>[2x]MGSSHHHHHHSSG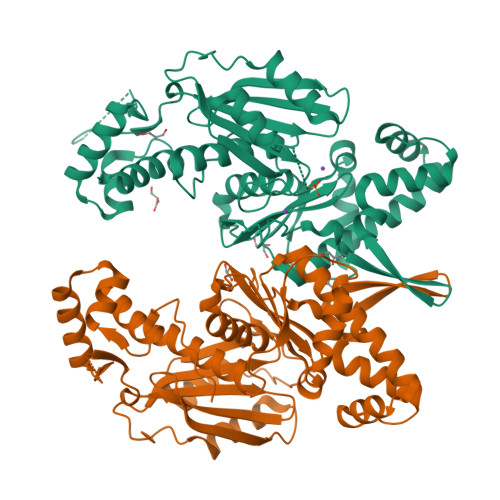ENLYFQGPMNDNEKRVLREIYNHHNISRTQISKNLEINKATISSILNKLKYKSLVNEVGEGDSTKSGGRKPILLKVNHLYGYFISLDLTYSSVEVMYNYFDGNVIKHESYDLPDEKVSSILSIIKKHIDIQEKLDTYNGLLGVSVSIHGVVDNEQHVTYLPFHETEGISIAKKIKEITNVPVVVENEANLSALYERNFNHNLSYNNLIALSIHKGIGAGLIINNQLYRGANGEAGEIGKTLVSKVSDNVEIFHKIEDIFSQEALLHNLSNQLNEKMTLSKLIQFYNEKNPVVVEEMEQFINKIAVLIHNLNTQFNPNAIYINCPLFNEMPEILEAIKNQFKQYSRNEIQIKLTSNVKFATLLGGTLAIIQKVLQINDIYLDIKA> DGVGNASGDWH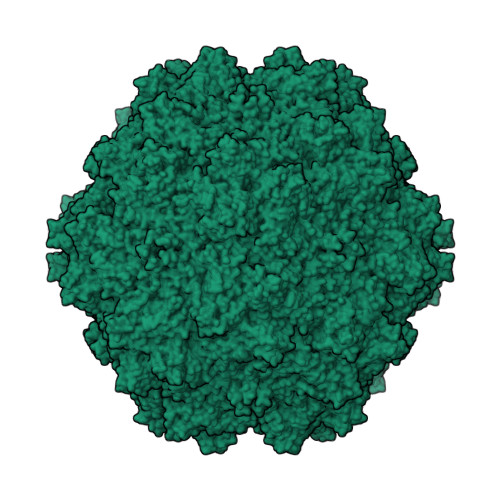CDSTWMGDRVVTKSTRTWVLPSYNNHQYREIKSGSVDGSNANAYFGYSTPWGYFDFNRFHSHWSPRDWQRLINNYWGFRPRSLRVKIFNIQVKEVTVQDSTTTIANNLTSTVQVFTDDDYQLPYVVGNGTEGCLPAFPPQVFTLPQYGYATLNRDNTENPTERSSFFCLEYFPSKMLRTGNNFEFTYNFEEVPFHSSFAPSQNLFKLANPLVDQYLYRFVSTNNTGGVQFNKNLAGRYANTYKNWFPGPMGRTQGWNLGSGVNRASVSAFATTNRMELEGASYQVPPQPNGMTNNLQGSNTYALENTMIFNSQPANPGTTATYLEGNMLITSESETQPVNRVAYNVGGQMATNNQSSTTAPATGTYNLQEIVPGSVWMERDVYLQGPIWAKIPETGAHFHPSPAMGGFGLKHPPPMMLIKNTPVPGNITSFSDVPVSSFITQYSTGQVTVEMEWELKKENSKRWNPEIQYTNNYNDPQFVDFAPDSTGEYRTTRPIGTRYLTRPL> GAGTMQPGATTC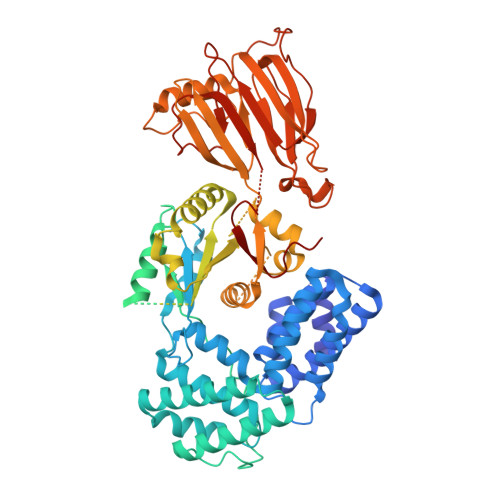TEDRIQHALERCLHGLSLSRRSTSWSAGLCLNCWSLQELVSRDPGHFLILLEQILQKTREVQEKGTYDLLAPLALLFYSTVLCTPHFPPDSDLLLKAARTYHRFLTWPVPYCSICQELLTFIDAELKAPGISYQRLVRAEQGLSTRSHRSSTVTVLLLNPVEVQAEFLDVADKLSTPGPSPHSAYITLLLHAFQATFGAHCDLSGLHRRLQSKTLAELEAIFTETAEAQELASGIGDAAEARQWLRTKLQAVGEKAGFPGVLDTAKPGKLRTIPIPVARCYTYSWNQDSFDILQEILLKEQELLQPEILDDEEDEDEEDEEEDLDADGHCAERDSVLSTGSAASHASTLSLASSQASGPTLSRQLLTSFVSGLSDGVDSGYMEDIEESAYERPRRPGGHERRGHRRPGQKFNRIYKLFKSTSQMVLRRDSRSLEGSPDSGPPLRRAGSLCSPLDSPTLPPSRAQRSRSLPQPKLSPQLPGWLLAPASRHQRRRPFLSGDEDPKASTLRVVVFGSDRISGKVARAYSNLRRLENNRPLLTRFFKLQFFYVPVKRSRGTGTPTSPAPRSQTPPLPTDAPRHPGPAELGAAPWEESTNDISHYLGMLDPWYERNVLGLMHLPPEVLCQSLKAEPRPLEGSPAQLPILADMLLYYCRFAARPVLLQVYQTELTFITGEKTTEIFIHSLELGHSAATRAIKASGPGSKRLGIDGDREAVPLTLQIIYSKGAISGRSRWSNMEKLCTSVNLSKACRQQEELDSSTEALTLNLTEVVKRQTPKSKKGFNQISTSQIKVDKVQIIGSNSCPFAVCLDQDERKILQSVIRCEVSPCYKPEKSSLCPPPQRPSYPPAPATPDLCSLLCLPIMTFSGALP>XNLAALRSELQALRREGFSPERLAALESRLQALERRLAALRSRLQALRGX[2x];>[2x]XGLCALRSELQALRREGFSPEELAALESELQALERE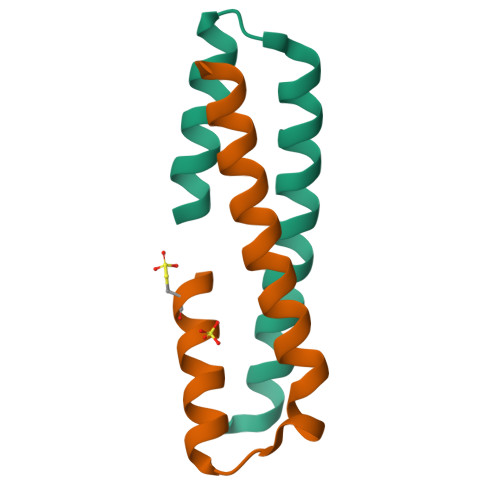LAALRSELQALRGX> MKTLIIETANAKILGELVTVSRLFGQAPDVVVLGSGELQGSYGKAYRLSDTLGANLGSSLSDLIKRERYELILLSTTAIGSGLAGPLAVSLGAPILSEVTAISPDLTIERSLYGSKAVARYKLESGPLVLTIKRKYFEAATLEGTTATEELPVGPQKITLLEEIEEERTGIPLEDAEVVVTGGRGIGSGDNFSILKEIAGMLNGAVGASRGAVDEGWMPPGAQIGQTGKIVAPTVYFAVGVSGASQH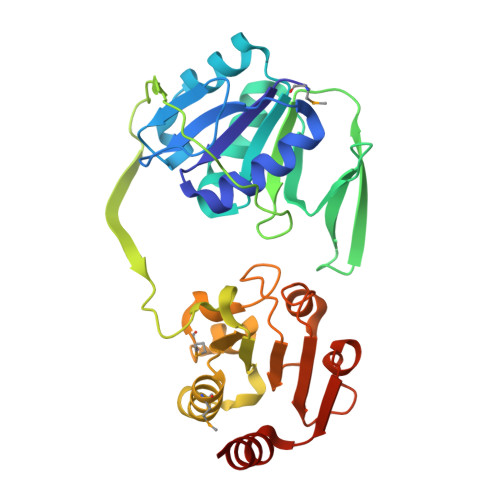LAGISNAKCVIAINKDNEANIFKRARFGIVGDYKKAVPALINALKEN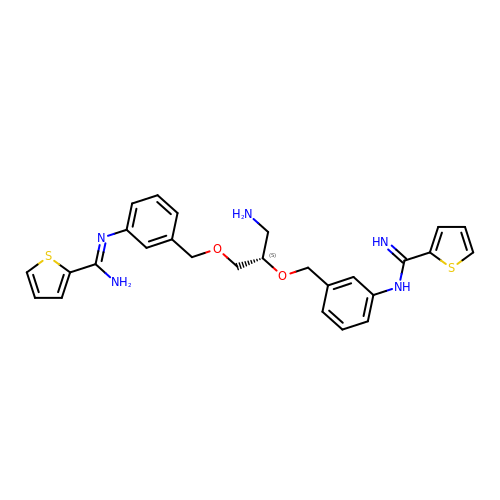N,N''-{[(2S)-3-aminopropane-1,2-diyl]bis(oxymethanediylbenzene-3,1-diyl)}dithiophene-2-carboximidamide | C27 H29 N5 O2 S2 | KEUPBLDQGUHFOB-QHCPKHFHSA-N>NPCCSHPCQNRGVCMSVGFDQYKCDCTRTGFYGENCSTPEFLTRIKLFLKPTPNTVHYILTHFKGFWNVVNNIPFLRNAIMSYVLTSRSHLIDSPPTYNADYGYKSWEAFSNLSYYTRALPPVPDDCPTPLGVKGKKQLPDSNEIVEKLLLRRKFIPDPQGSNMMFAFFAQHFTHQ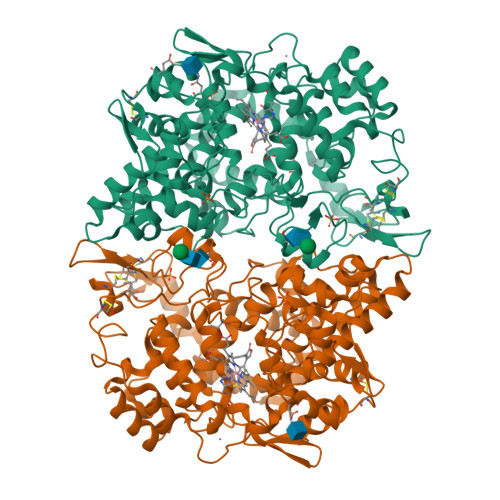FFKTDHKRGPAFTNGLGHGVDLNHIYGETLARQRKLRLFKDGKMKYQIIDGEMYPPTVKDTQAEMIYPPQVPEHLRFAVGQEVFGLVPGLMMYATIWLREHNRVCDVLKQEHPEWGDEQLFQTSRLILIGETIKIVIEDYVNHLSGYHFKLKFDPELLFNKQFQYQNRIAAEFNTLYHWHPLLPDTFQIHDQKYNYQQFIYNNSILLEHGITQFVESFTRQIAGRVAGGRNVPPAVQKVSQASIDQSRQMKYQSFNEYRKRFMLKPYESFEELTGEKEMSAELEALYGDIDAVELYPALLVEKPRPDAIFGETMVEVGAPFSLKGLMGNVICSPAYWKPSTFGGEVGFQIINTASIQSLICNNVKGCPFTSFSVP[2x]> GSHMMPGEIRPTIGQQMETGDQRFGDLVFRQLAPNVWQHTSY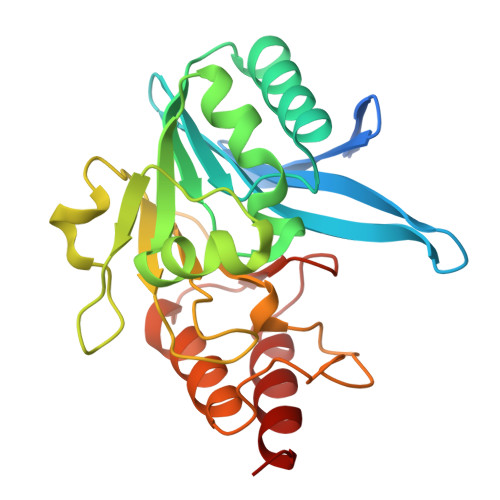LDMPGFGAVASNGLIVRDGGRVLVVDTAWTDDQTAQILNWIKQEINLPVALAVVTHAHQDKMGGMDALHAAGIATYANALSNQLAPQEGMVAAQHSLTFAANGWVEPATAPNFGPLKVFYPGPGHTSDNITVGIDGTDIAFGGCLIKDSKAKSLGNLGDADTEHYAASARAFGAAFPKASMIVMSHSAPDSRAAITHTARMADKLR>GPLGSPGIPGKEILRNPMEAMDPHIFYFHFKNLRKAYGRNESWLCFTMEVVKHHSPVSWKRGVFRNQVDPETGRHAERCFLSWFADDILSPNTNYEVTWYTSWSPCPECAGEVAEFLARHSNVNLTIKTARLYYFDDTDYQEGLRSLSQE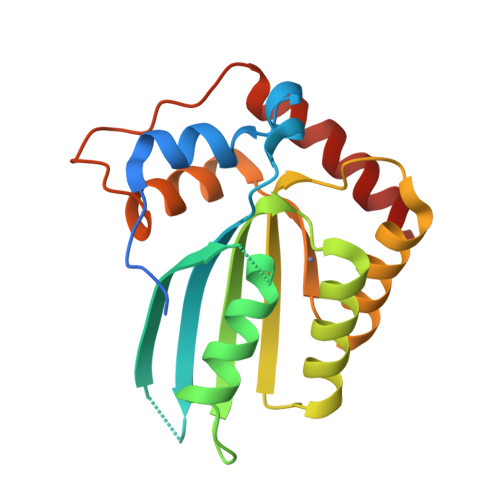GASVEIMGYKDFKYCWENFVYNDDEPFKPWDGLDYNFLDLDSKLQEILE[2x]>[2x]MGDNEKINREALAPREYGESLELGIEFTTTEEIEVPEKLIDQVIGQEHAVEVIKTAANQKRHVLLIGEPGTGKSMLGQAMAELLPTETLEDILVFPNPEDENMPRIKTVPACQGRRIVEKYREKAKS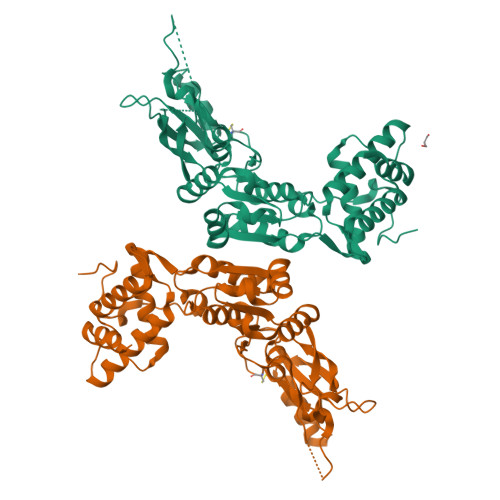QESVKSYILLFVMFTVMLALFIEFSATTLLMGLFVVILTIMALSNMRLKSTVLVPKLLVDNCGRTKAPFIDATGAHAGALLGDVRHDPFQSGGLGTPAHERVEPGMIHRAHKGVLFIDEIATLSLKMQQSLLTAMQEKKFPITGQSEMSSGAMVRTEPVPCDFVLVAAGNLDTVDKMHPALRSRIRGYGYEVYMRTTMPDTIENRRKLVQFVAQEVKRDGKIPHFTKEAVEEIVREAQKRAGRKGHLTLRLRDLGGIVRAAGDIAVKKGKKYVEREDVIEAVKMAK(2E)-N-ALLYL-4-{[3-(4-BROMOPHENYL)-5-FLUORO-1-METHYL-1H-INDAZOL-6-YL]OXY}-N-METHYL-2-BUTEN-1-AMINE 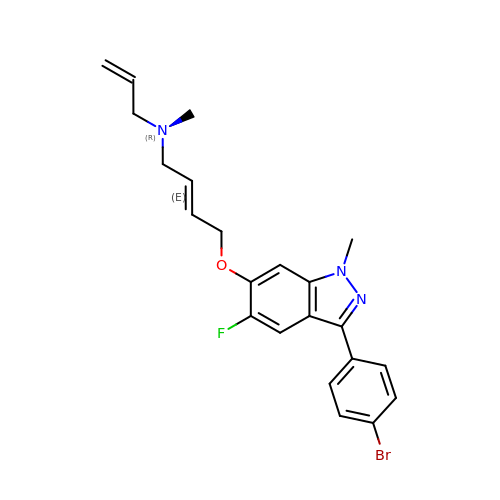| C22 H23 Br F N3 O | YDWPQZUWZDRRSE-AATRIKPKSA-N> MTLYRLHEADLEIPDAWQDQSINIFKLPASGPAREASFVISRDASQGDAPFADYVARQLENAEKQLPGFKLHKRW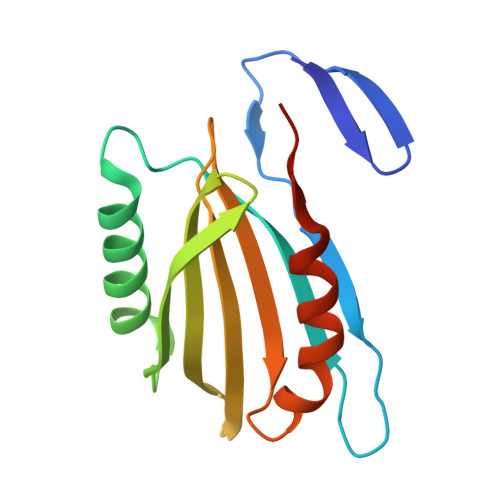DINIHGHAAVLLDYQWQREGRDLMLRQVFIERRPAVLITTLTTTPADLPHHEPAWKQAMQTLVPRPTPSGS>SGWVWNQFFVIEEYTGPDPVLVGRLHSDIDSGDGNIKYILSGEGAGTIFVIDDKSGNIHATKTLDREERAQYTLMAQAVDRDTNRPLEPPSEFIVKVQD[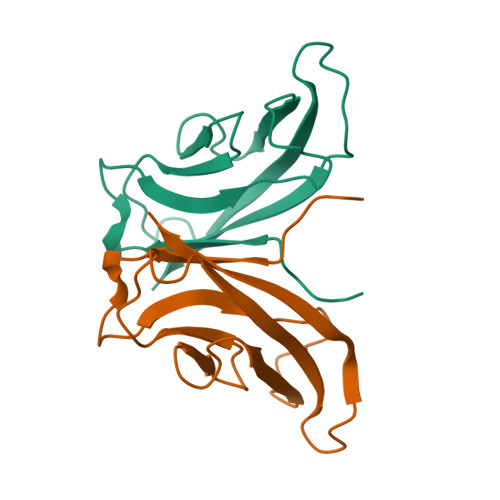2x]> ADLPAPDDTGLQAVLHTALSQG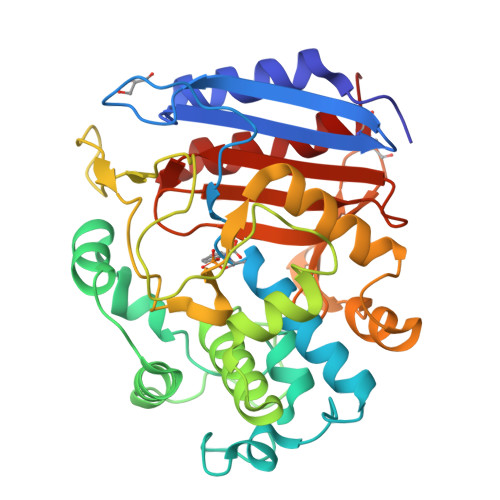APGAMVRVDDNGTIHQLSEGVADRATGRAITTTDRFRVGSVTKSFSAVVLLQLVDEGKLDLDASVNTYLPGLLPDDRITVRQVMSHRSGLYDYTNDMFAQTVPGFESVRNKVFSYQDLITLSLKHGVTNAPGAAYSYSNTNFVVAGMLIEKLTGHSVATEYQNRIFTPLNLTDTFYVHPDTVIPGTHANGYLTPDEAGGALVDSTEQTVSWAQSAGAVISSTQDLDTFFSALMSGQLMSAAQLAQMQQWTTVNSTQGYGLGLRRRDLSCGISVYGHTGTVQGYYTYAFASKDGKRSVTALANTSNNVNVLNTMARTLESAFCGKP> MSKPQNNDTLELDDILSQPVKDKERFAAFMMRKLAENKPAQNDNLFGNFKLDFDLDFEVPLIKKSQAKPKSKLPEVQPLGELVSKNSAATEKVNEPPVDQAPNENVPPRRSPTLSPNNRRSMRRSGNVPGSDKLRRHAIRRRSRSCGRQLLPEFEETVNLTRSISSPVNFLPEISSTPCTEKQKEEVAKNTTRVETDKPAEKPMELSQEPEPENPLQTKVTSPARNPILAAEIEQICKERQSSFHKNVLQLDYSGRAPYSRPPTPSSPSVAGLRRTYTMEKGPAPGQLLLSPSHRYDTPSKMPVVKAKRFNQELMVPDTPERQSHDPAWQSEPQPEFVVPETQPQDLGELVQTLSRSAISPIVVINTSNSNRSVRRDAVAMKSVPTSPVTALSSPPIAPSPRRSAAASPQKSIAQLPRVEENMDAIMTDDESDEHPSTVPLNLAPSGGNTTRQRRLRSSNRARATIESQESSMRLLNLHKSVNAKKSKPRKTAIPLNKAPSAPINGEQFARELTRMSNYEILDLRKRNSLNEIYPLNGHRNHRSEKLILEEEIQRELLRRNLMDEAEGLPKQQSSDDSNEDYIPVPPKTQSLRTKSNDRSQGRGRPRSTRRDLPMTTELVNYLGLSQTLETRRKSSKDGKRCLYTKGSSDHEDNDSLSPVKLPRLSKS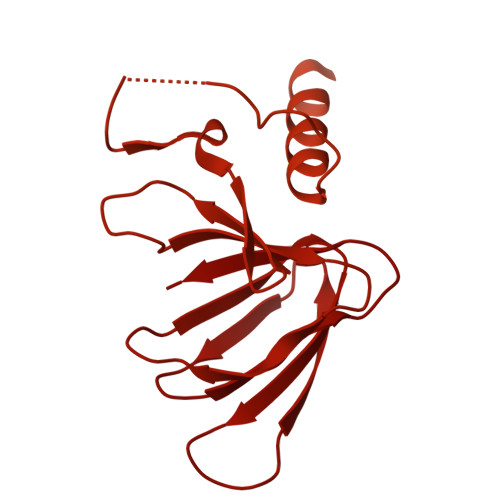IQIVPPPPVSLRYSQSLQNLPCSGKFDFDNVVMAAPPDFHDSVNSDAIEIAPPPPEYVVNTRGRSTSGRKSNKNDLVLPPPGYEGGQEEEHDERPSQPRCTAKELQQSTQNGRRAMENELVPPPIEYVEEENRNNEQSRRSTKNGNLVDRNTHNAVEYCEPPEPPEYDDSDHGQASILRRSGKKLQHSKQSVQKSNKEQIIAPSYENNEDYDSDEEPIYNEEYGKEESQNKNVTRRKSDKDEMASHTLECIEGPDPNWNSSCNKQNRNHQNASKSKENDKLANRSSKSQKLSNPRQNAVGTEKSVALSNRGEECTEKSSDVMESLRVNTPTPPIDQNSDDVPSRNPSPSRTLLSDDVPSTSRAALEFLQRSQNMSKSRPPDESSADVVFKKPLAPAPRAKSKKGKSEVDKLKLAKMPVEAEELNTTGIRRSKRGQVPLQMSWCHTMDPSKFNFMSGFIEPRSKNSKTKKGNLSKAKKASATKPKPTVEKNLPDNRGPLCSSTPRISEKLPGAIPHSESLGLSTLTWEETEVQAEAEKVPKKRGRPKKAVGGVQTDTEAEPEPEPEPMISSVAPLTSDQEEPDVPDEQAPYTEAALGPVVFSTPLRDEQEEASTKLMQWLRGVGDAPPSASMSDENASVSSANELIFYQVDGIDYAFYNTKEKAMLGYMRFKPYQKRSMKQAKVHPLKLLVQFGEFNVETLAVGEEKEVHSVLRVGDMIEIDRGTRYSIQNAIDKVSVLMCIRS>[2x]SLLNVPAGKDLPEDIYVVIEIPANADPIKYEIDKESGALFVNRFMSTAMFYPCNYGYINHTLSLDGDPVDVLVPTPY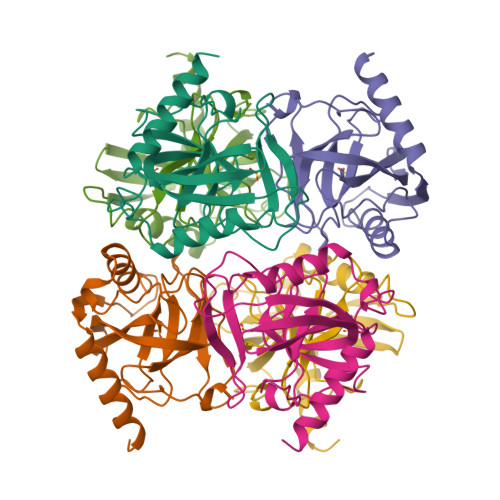PLQPGSVIRCRPVGVLKMTDEAGEDAKLVAVPHSKLSKEYDHIKDVNDLPELLKAQIAHFFEHYKDLEKGKWVKVEGWENAEAAKAEIVASFERAKNK> AKALIVYGSTTGNTEYTAETIARELADAGYEVDSRDAASVEAGGLFEGFDLVLLGCSTWGDDSIELQDDFIPLFDSLEETGAQGRKVACFGCGDSSHEYFCGAVDAIEEKLKNLGAEIVQD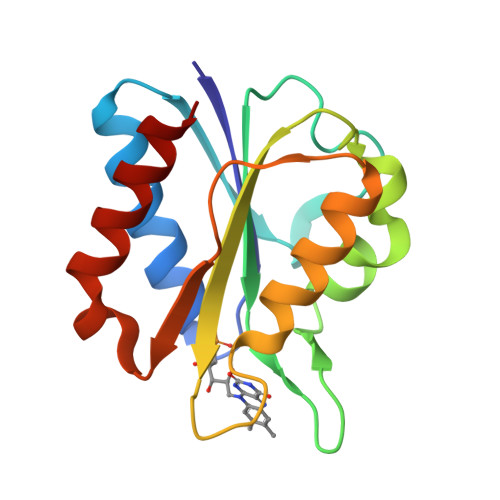GLRIDGDPRAARDDIVGWAHDVRGAI> GPLGSPEFNRPVKRMIALYDYDPQELSPNVDAEQVELCFKTGEIILVYGDMDEDGFYMGELDGVRGLVPSNFLAD;> XIGRRLPPTPSKPSTLX

RBP, via its second and third SH3 domain, is known to bind synaptic ligands such as Ca2+ channels and RIM. Drosophila RBP SH3-II and -III share 49.2% sequence identity and adopt the canonical fold of SH3 domains. We observed the classical poly-proline helix that allows for mainly hydrophobic protein-peptide interaction in all three structures. In summary, we find that the SH3-II and -III interaction surface of RBP serves as a multi-functional platform for differential protein interaction with either other AZ components or the transport adaptor and therefore, motor-cargo linkage.

Finally, in order to get a deeper atomic insight into the structural basis of the binding of RBP towards Aplip1 in comparison to its synaptic ligands, we crystallized the Drosophila RBP SH3-II domain together with both an Aplip1 and a Cac peptide, and RBP SH3-III with a Cac peptide. The Cac-derived peptide bound to SH3-III is fully defined in the electron density. However, the peptide main chain interaction with the SH3 domains is conserved. The side chain orientation of Cac R1687 is again different if bound to SH3-II or SH3-III. In complex with SH3-III, R1687 forms a bidentate hydrogen bond to SH3-III D1463 and E1648. A π-stacking interaction is not possible since Y1372 of SH3-II is replaced by SH3-III L1499.> ANVPTGVQLAEKQVLVRNNGSEPQSLDPHKIEGVPESNISRDLLEGLVINDPNGNIVPGAAESWDNKDFKVWTFNIRKDAKWSNGDPVTAQDFVYSWQRLADPKTVSPYASYLQYAHLTNIDDIITGKAAPDTLGVKALDDHTLEVTLSEPVPYLDKLLAHPLMSPVNKTVVEKFGEKWTQPQNFVGNGAYKLKDWIVNERIVLERSPTYWDNAKTVINQVTYLPISSEVTDVNRYRSGEIDMTYNNMPIELFQKLKKEIPDQVHVDPYLCTYYYEINNQKAPFTDARVREALKLGMDRDIIVNKVKNQGDLPAYGFTPPYTSGAELTPPEWFSWTQEKRNEVAKKLLAEAGYTKDNPLKFSLLYNTSDLHKKLAIAAASIWKKNLGVDVKLENQEWKTFLDTRHQGTYDVARAAWCADYNEPSSFLNMMLSNSSNNTTHYKSSVFDKLIEDTLKVKSEKERADLYQQAEIQLDKDSAIVPVFYYV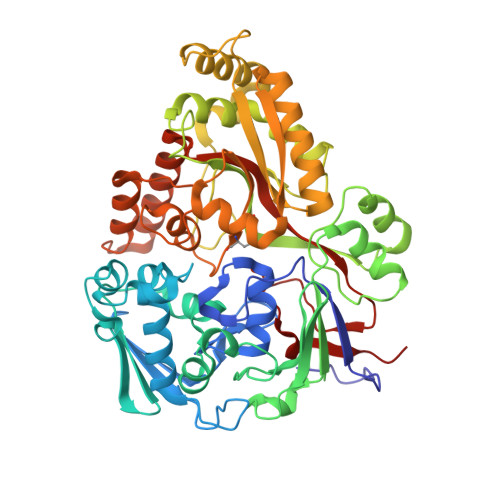SARLVKPYVGGYTGKDPLDNMHVKDLYIIKQ> MSLLEGLALFLLLLSGVLVVTLRNAIHAALALILNFLVLAGVYVALDARFLGFIQVIVYAGAIVVLFLFVIMLLFAAQGE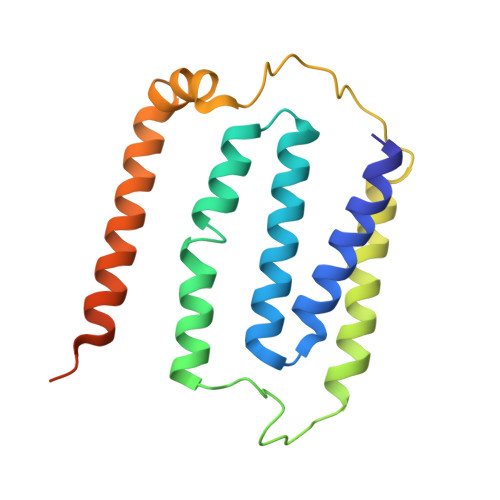IGFDPLVRSRPLAALLALGVAGILAAGLWGLDLAFTQDLKGGLPQALGPLLYGDWLFVLLAVGFLLMAATVVAVALVEPGKASRAKEAEKREEVAR>GSSGEGQKDLKLGELLLQKGWISREALEEALVEQEKTGDLLGRILVRKGLPEEALYRALAEQKGLEFLESTEGIVPDPSAALLLLRSDALRYGAVPIGFQNGEVEVVLSDPRHKEAVAQLLNRPARFYLALPQAWEELFRRAYPQK[2x]

The traffic ATPase PilF from Thermus thermophilus is important for type IV pilus biogenesis, twitching motility, surface attachment, and natural DNA-uptake and contains three consecutive homologous GPSII domains. The N-terminal part of PilF harbors a remarkable arrangement of three successive general secretory pathway II (GSPII) domains (GSPII-A to GSPII-C) with high sequence similarity to each other. Interestingly, we find that PilF binds only two molecules of c-di-GMP with different affinities and that the c-di-GMP–binding activities can be attributed to the GSPII-B and GSPII-C domains. Remarkably, the GSPII-B domain binds c-di-GMP with a KD of only 6 nM and thus with an affinity ∼ 83fold higher than MshEN.

The crystal structure of PilF159–302 in complex with c-di-GMP was determined by molecular replacement using the NMR-solution structure of c-di-GMP–bound PilF159–302 as a starting point. The crystals diffracted to ∼2 Å and the protein chain could be traced without interruption from residue 165 to 301 with c-di-GMP fitting perfectly into the difference electron density. The N-terminal subdomain spans residues 167 to 221 and consists of a tightly packed four helix bundle in which helix α1 and α2 as well as α3 and α4 are parallel to each other. The C-terminal subdomain exhibits a fold in which a mixed four-stranded β-sheet at the core of the subdomain is surrounded by four helices and the inflexible linker. In sum, the PilF159-302 structure consists of eight α-helices and four β-strands which is consistent with the previously derived secondary structure. c-di-GMP is bound in an elongated, slightly bulged conformation to the N-terminal subdomain with only the amino group of one of the guanine bases oriented towards the C-terminal subdomain. The 10 direct intermolecular hydrogen bonds identified between the N-terminal subdomain of PilF159-302 and c-di-GMP are all conserved in comparison to the intermolecular hydrogen bonds described for MshEN, highlighting the importance of these conserved residues for the MshEN-like c-di-GMP–binding mode. The N-terminal hydrophobic cluster is formed by L183 and L187 from motif I and L197 from motif II while L168 from motif I and L211 and L215 from motif II form the C-terminal hydrophobic cluster. Inspection of the presented X-ray and NMR-structures of PilF159-302 in complex with c-di-GMP shows that these two residues are involved in extensive hydrophobic stacking interactions with the two guanine bases. The sidechain of K167 extends diagonally across the GMP1 guanine base plane with its hydrophobic region (Cβ to Cε methylene groups) located on top of the guanine base. Furthermore, the cationic amino group of K167 is in a position enabling a cation-π-interaction in addition to the hydrophobic stacking.Btk is critical for the generation of calcium flux in response to receptor activation, because it activates phospholipase C-γ2 (PLC-γ2), which produces the second messengers diaceylglycerol (DAG) and inositol (1,4,5)-trisphosphate (IP3). Btk dysfunction is the cause of X-linked agammaglobulinemia, a severe disease of primary immunodeficiency. The Tec family kinases have a lipid-interaction module attached to the N terminus of a Src-like module (i.e., concatenation of an SH3 domain, an SH2 domain and a tyrosine kinase domain). The lipid-interaction module of the Tec kinases is an extended plekstrin homology (PH) domain fused to a Tec homology (TH) domain.

We determined a crystal structure of the Btk PH-TH module bound to IP6 at 2.3 Å. There are four PH-TH modules in the asymmetric unit of the crystal, which form two dimers, similar to those seen in other structures of the Btk PH-TH module. The four PH-TH modules in the asymmetric unit have six bound IP6 molecules, each with clearly resolved electron density. Four of the IP6 molecules are in the canonical binding sites on each module. At those sites, residues Asn 24, Tyr 39, Arg 28, and Lys 12 coordinate phosphate groups on the 2, 3, and 4 positions of the myo-inositol ring; these are also the key residues involved in IP4 binding. The two other IP6 molecules in the crystallographic asymmetric unit are bound at a peripheral site. This site is on the surface formed by an elongated β hairpin involving strands β3 and β4 of each PH-TH module. Residues Arg 49, Lys 52, Lys 36, and Tyr 40 at the peripheral binding site of one subunit coordinate phosphate groups at the 1, 2, 3, and 4 positions of the myo-inositol ring. The Saraste dimer is formed by symmetric interactions between helix α1 and strands β3 and β4 of the PH-TH module.

>GMATVILESIFLKRSQQKKKTSPLNFKKRLFLLTVQKLSYYEYDFERGRRGSKKGSIDVEKITCVETVVPEKNPPPERQIPRRGEESSETEQISIIERFPYPFQVVYDEGPLYVFSPTEELRKRWIHQLKNVIRYNSDLVQKYHPCFWIDGQYLCCSQTAKNAMGCQILEN[4x]First reported in 19541, protein tyrosine O-sulfation (PTS) entails the transfer of a sulfate group from 3′-phosphoadenosine 5′-phosphosulfate (PAPS) to a protein tyrosine residue under the catalysis of membrane-bound tyrosylprotein sulfotransferases (TPSTs) in the trans-Golgi. To meet above challenges, the genetic incorporation of sTyr into proteins in response to amber nonsense codon (TAG) was reported. Here we report the synthesis of site-specifically sulfated proteins in both live yeast and mammalian cells through the genetic incorporation of sTyr using an engineered tyrosyl-tRNA synthetase derived from E. coli (EcTyrRS). In order to understand the shifted substrate specificity, we obtain a crystal structure of the evolved sTyrRS in complex with sTyr, which also shed lights on future engineering of the enzyme for substrates with similar physicochemical properties.

We obtained and refined the crystal structure of the evolved sTyrRS in complex with sTyr at 1.78 Å resolution. The protein formed a homodimer, the same as the wild-type EcTyrRS. In addition, the D182G mutation eliminates the potential repulsion between the negatively charged carboxylate group of Asp and the sulfate group of sTyr. This mutation also contributed to the lowered affinity of the evolved sTyrRS towards Tyr, due to the abolishment of a stabilizing hydrogen bond. A third mutation, W129F, contributes to the substantially lower background activity of the c2 variant towards Tyr. This is likely due to the smaller size of the Phe side chain, which further contributes to the enlarged active site. A close inspection of ligand binding revealed that the phenol ring of the sTyr tilted around 26° away from that of the Tyr. This movement enabled the formation of a hydrogen bond between the sulfate group and the hydroxyl group of Tyr37 residue. Since this Tyr is also critical for the binding of Tyr substrate in the active site of the wild-type EcTyrRS, its retention likely played a major role in the background activity of the evolved sTyrRS towards Tyr when sTyr was not available. Another key interaction that anchors the sulfate group is a hydrogen bond with the side chain of Asn126, which does not participate in substrate binding in the wild-type EcTyrRS.

>[2x]MASSNLIKQLQERGLVAQVTDEEALAERLAQGPIALYCGFDPTADSLHLGHLVPLLCLKRFQQAGHKPVAVVGGATGLIGDPSFKAAERKLNTEETVQEWVDKIRKQVAPFLDFDCGENSAIAANNYDFFGNMNVLTFLRDIGKHFSVNQMINKEAVKQRLNREDQGISFTEFSYNLLQGYGFACLNKQYGVVLQIGGSDQWGNITSGIDLTRRLHQNQVFGLTVPLITKADGTKFGKTEGGAVWLDPKKTSPYKFYQFWINTADADVYRFLKFFTFMSIEEINALEEEDKNSGKAPRAQYVLAEQVTRLVHGEEGLQAAKR> LRSIHHLIASHRRLFKFIRHYTINKMKSALIATALLAGSAAAFTSNAGSQSTSALKAMPERLWDSMVDKTERSKAVPFLPRAVNLDGSLPGDVGFDPFYLSSIPKDFSGFIQPPQWEEKGIPTLYWMREAELKHCRVAMLAWFGWLATDGAFGVTLRFPGEIYSVENIPTA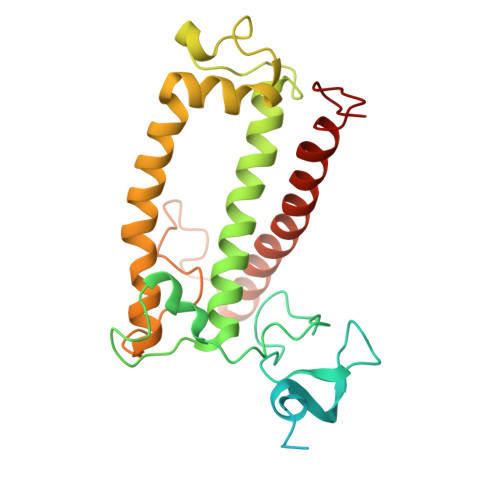YEAHNALVSQGSMGFLLLAVGFIEFCTGAVLVEVAKGASDREAGDFKLDPLSFLKGKSEEEIKRMKTREIANGRLAMLAFGGVATQTALEGGNHAFPYF>SVDLIGINVAGAEFTGGKLPGKHGTHYFFPPEGYFEYWSEQGIHTVRFPLKWERLQPSLNAELDDVYASLVDDMLDQAKENDIKVILDVHNYARYRKKVIGTEDVPVSAYQDLMERIAKRWQGHDALFAYDIMNQPYGSADKLWPAAAQAGIDGVRKYDKKRPLLIEGASWSSAARWPRYADELLKLKDPADNMVFSAHVYIDEDASGSYKKGPGKDFEPMIGVKRVEPFVNWLKEHGKKGHIGEFGIPNDDERWLDAMDKLLAYLNENCIPINYWAAGPSWGNYKLSIEPKDGEKRPQVALLKKYAAKDNCSDFGPAKAE[2x]

RBcel1, an endoglucanase of the GH5_5 subfamily isolated from an uncultured bacterium, has aroused interest because of its ability to polymerize cellooligosaccharides in vitro under near-physiological conditions. After the glycosylation step, the donor sugar is covalently bound to the enzyme within its negatively numbered subsites. Transglycosylation occurs when a sugar hydroxyl group is used as an acceptor instead of a water molecule during the deglycosylation step. Solving the structures of two RBcel1 variants, RBcel1_E135Q and RBcel1_Y201F, in complex with ligands has brought to light some of the molecular factors behind transglycosylation.

Thus, to mimic the presence of the GluA/B residue, the variant RBcel1_E135Q was generated to determine its structure with G3. The activity of this variant was dramatically impaired with ClPNP β-G3 as substrate, with a k cat of 0.219 ± 0.009 × 10−3 min−1 and a K m of 0.263 ± 0.041 mM. The kinetic parameters strongly indicate that both the glycosylation and deglycosylation steps are affected by the substitution of Glu135 with a glutamine residue. The side chain of the nucleophile Glu245 is positioned as described for RBcel1_WT in monomer A and the apo form of RBcel1_E135Q. The mt-10° to tt0° rotation seems to impact the position of the side chain of Tyr201. When Glu245 adopts the tt0° conformation, as seen in monomer B, the hydroxyl group of Tyr201 is displaced by 1 Å compared with monomer A and the apo form of RBcel1_E135Q.> GAGSMKKLLNTLYVTQPDTYLSLDGDNVVLLKEQEKLGRLPLHNLEAIVGFGYTGASPALMGYCAERNISITFLTKNGRFLARVVGESRGNVVLRKTQYRISENDQESTKIARNFITGKVYNSKWMLERMTREHPLRVNVEQFKATSQLLSVMMQEIRNCDSLESLRGWEGQAAINYNKVFDQMILQQKE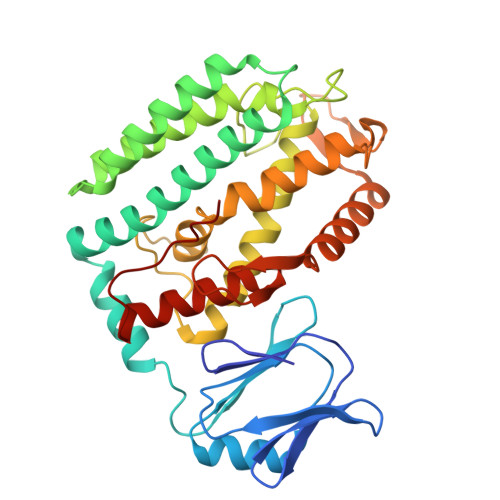EFAFHGRSRRPPKDNVNAMLSFAYTLLANDVAAALETVGLDAYVGFMHQDRPGRASLALDLMEELRGLYADRFVLSLINRKEMTADGFYKKENGAVLMTDEARKTFLKAWQTKKQEKITHPYLGEKMSWGLVPYVQALLLARFLRGDLDEYPPFLWK>SHMRIVFDIGGSVLVPENPDIDFIKEIAYQLTKVSEDHEVAVVVGGGKLARKYIEVAEKFNSSETFKDFIGIQITRANAMLLIAALREKAYPVVVEDFWEAWKAVQLKKIPVMGGTHPGHTTDAVAALLAEFLKADLLVVITNVDGVYTADPK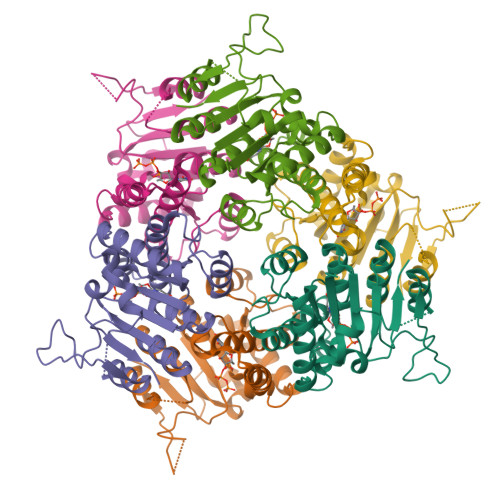KDPTAKKIKKMKPEELLEIVGKGIEKAGSSSVIDPLAAKIIARTGIKTIVIGKEDAKDLFRVIKGDHNGTTIEP[2x]>MEDLQKALEAQSRALRAELAAGASQSRRPRPPRQRDSSTSGDDSGRDSGGPRRRRGNRGRGQRRDWSRAPPPPEERQETRSQTPAPKPSRAPPQQPQPPRMQTGRGGSAPRPELGPPTNPFQAAVARGLRPPLHDPDTEAPTEACVTSWLWSEGEGAVFYRVDLHFTNLGTPPLDEDGRWDPALMYNPCGPEPPAHVVRAYNQPAGDVRGVWGKGERTYAEQDFRVGGTRWHRLLRMPVRGLDGDSAPLPPHTTERIETRSARHPWRIR[2x]

Rubella virus is an enveloped, positive-stranded RNA virus with virions ranging from 500 Å to 900 Å in diameter. The structural components of rubella virus are comprised of three proteins, glycoproteins E1 (58kDa), E2 (42–47kDa), and the capsid protein (31kDa). In this report, we have used a combination of cryo-electron tomography, sub-tomogram averaging and in vitro assembly studies to elucidate the three-dimensional structure and assembly of rubella virions. Instead, the structure of rubella virus, as shown here, has an irregular helical organization of its surface glycoproteins and a pseudo-tetrameric inner nucleocapsid arrangement.

The third structural protein of rubella virus is the capsid protein, which interacts via its amino-terminal domain with the viral RNA genome to form the inner nucleocapsid. The atomic structure of the carboxy-terminal domain of the capsid protein is known and presumably forms the structural framework of the viral nucleocapsid. The cryo-electron density from about 20 isolated tetrameric units seen in the tomograms of the in vitro assembled nucleocapsid cores were re-oriented to a common orientation and averaged. This showed that each monomer of the tetrameric unit has a dumbbell-shaped structure. The structure of the C-terminal domain of the capsid protein dimer was fitted into one lobe of the dumbbell shaped averaged density of the in vitro assembled nucleocapsid tetramers using the EMfit program. The two top fitting orientations for the capsid protein in the averaged density are 180° apart, relative to each other, along an axis perpendicular to the two-fold axis of the capsid dimer. These best fitting conformations of the capsid protein are similar to the orientations of the capsid protein expected to be facing the viral membrane. As the N- and C-terminal domains of rubella capsid protein are similar in size, the remaining density of the averaged dumbbell shaped unit must be the location of the N-terminal domain of the capsid protein. Using these fitting results, it can be deduced that the disordered residues at the C-terminal end of the capsid protein, not seen in its crystal structure, likely correspond to the thin strips of density visible in the cross-section of rubella virion tomograms, linking the inner nucleocapsid shell to the membrane anchored E2 signal peptide in the viral membrane. The dumbbell shape of the capsid protein also accounts for the double-layer appearance seen in the in vitro nucleocapsids.> GPGSMKLVTVIIKPFKLEDVREALSSIGIQGLTVTEVKGFGRQKGHAELYRGAEFSVNFLPKVKIDVAIADDQLDEVIDIVSKAAYTGKIGDGKIFVAELQRVIRIRTG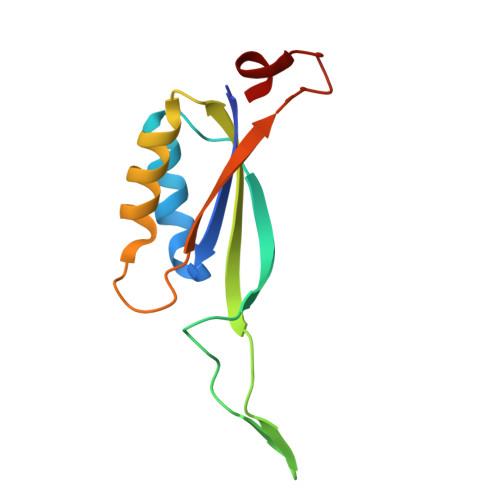EADEAAL> KPFKCSMCDYASVEVSKLKRHIRSHTGERPFQCSLCSYASRDTYKLKRHMRTHSGEKPYECYIC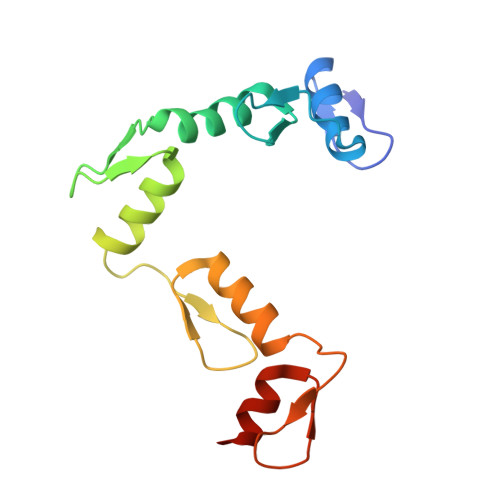HARFTQSGTMKMHILQKHTENVAKFHCPHCDTVIARKSDLGVHLRKQHSYIEQGKKCRYCDAVFHERYALIQHQKSHK>MASHHHHHHSGMTWLEPQIKSQLQSERKDWEANEVGAFLKKAPERKEQFHTIGDFPVQRTYTAADIADTPLEDIGLPGRYPFTRGPYPTMYRSRTWTMRQIAGFGTGEDTNKRFKYLIAQGQTGISTDFDMPTLMGYDSDHPMSDGEVGREGVAIDTLADMEALLADIDLEKISVSFTINPSAWILLAMYVALGEKRGYDLNKLSGTVQADILKEYMAQKEYIYPIAPSVRIVRDIITYSAKNLKRYNPINISGYHISEAGSSPLQEAAFTLANLITYVNEVTKTGMHVDEFAPRLAFFFVSQGDFFEEVAKFRALRRCYAKIMKERFGARNPESMRLRFHCQTAAATLTKPQYMVNVVRTSLQALSAVLGGAQSLHTNGYDEAFAIPTEDAMKMALRTQQIIAEESGVADVIDPLGGSYYVEALTTEYEKKIFEILEEVEKRGGTIKLIEQGWFQKQIADFAYETALRKQSGQKPVIGVNRFVENEEDVKIEIHPYDNTTAERQISRTRRVRAERDEAKVQAMLDQLVAVAKDESQNLMPLTIELVKAGATMGDIVEKLKGIWGTYRETPVFGSAWSHPQFEK[2x];>MASHHHHHHSGMDQTPIRVLLAKVGLDGHDRGVKVVARALRDAGMDVIYSGLHRTPEEVVNTAIQEDVDVLGVSLLSGVQLTVFPKIFKLLDERGAGDLIVIAGGVMPDEDAAAIRKLGVREVLLQDTPPQAIIDS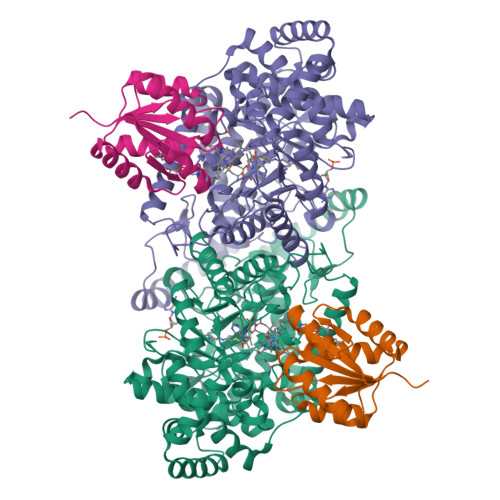IRSLVAARGARGSAWSHPQFEK[2x]>[2x]AQPAARDLKVVTKRGSADGCTDWSVDIKKYQ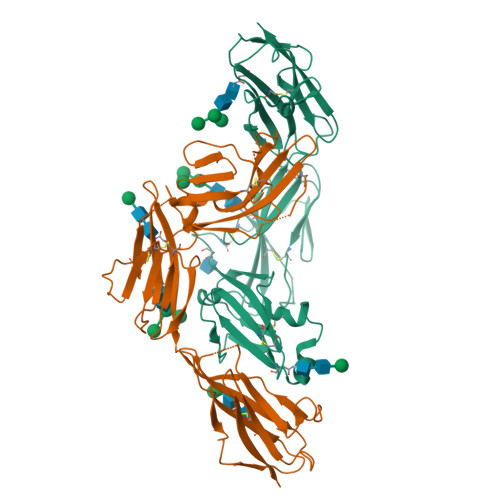VLVGEPVRIKCALFYGYIRTNYSLAQSAGLSLMWYKSSGPGDFEEPIAFDGSRMSKEEDSIWFRPTLLQDSGLYACVIRNSTYCMKVSISLTVGENDTGLCYNSKMKYFEKAELSKSKEISCRDIEDFLLPTREPEILWYKECRTKAWRPSIVFKRDTLLIKEVKEDDIGNYTCELKYGGFVVRRTTELTVTAPLTDKPPKLLYPMESKLTVQETQLGGSANLTCRAFFGYSGDVSPLIYWMKGEKFIEDLDENRVWESDIRILKEHLGEQEVSISLIVDSVEEGDLGNYSCYVENGNGRRHASVLLHKRKHHHHHH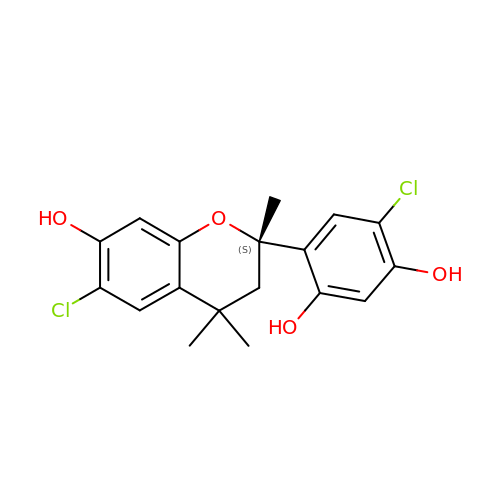4-chloranyl-6-[(2~{S})-6-chloranyl-2,4,4-trimethyl-7-oxidanyl-3~{H}-chromen-2-yl]benzene-1,3-diol | C18 H18 Cl2 O4 | VSHLILKLIDPGCI-SFHVURJKSA-N> GGSGGSGGSGGSGGSPTNYEYDEASETWPSFILTGLLMVVGPMTLLQIYQIFFGANAEDGNSGKSKEFNEEVFKNLNEEYTSDEIKQFRRKFDKNSNKKSKIWSRRNIIIIVGWILVAILLQRINSNDAIKDAATKLFDPYEILGISTSASDRDIKSAYRKLSVKFHPDKLAKGLTPDEKSVMEETYVQITKAYESLTDELVRQNYLKYGHPDGPQSTSHGIALPRFLVDGSASPLLVVCYVALLGLILPYFVSRWWARTQSYTKKGIHNVTASNFVSNLVNYKPSEIVTT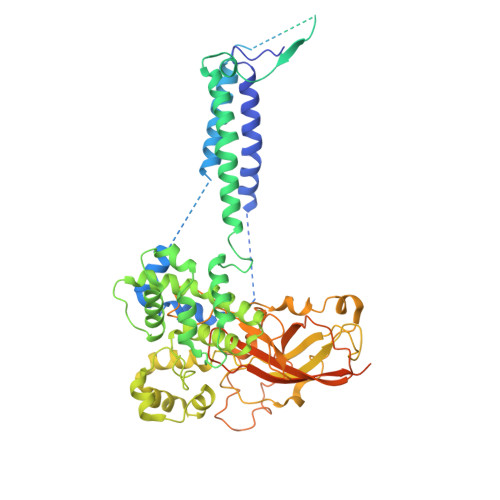DLILHWLSFAHEFKQFFPDLQPTDFEKLLQDHINRRDSGKLNNAKFRIVAKCHSLLHGLLDIACGFRNLDIALGAINTFKCIVQAVPLTPNCQILQLPNVDKEHFITKTGDIHTLGKLFTLEDAKIGEVLGIKDQAKLNETLRVASHIPNLKIIKADFLVPGENQVTPSSTPYISLKVLVRSAKQPLIPTSLIPEENLTEPQDFESQRDPFAMMSKQPLVPYSFAPFFPTKRRGSWCCLVSSQKDGKILQTPIIIEKLSYKNLNDDKDFFDKRIKMDLTKHEKFDINDWEIGTIKIPLGQPAPETVGDFFFRVIVKSTDYFTTDLDITMNMKVRDSPAVEQVEVYSEEDDEYSTDDDETESDDESDASDYTDIDTDTEAEDDESPEAGGATTASGTGENLYFQ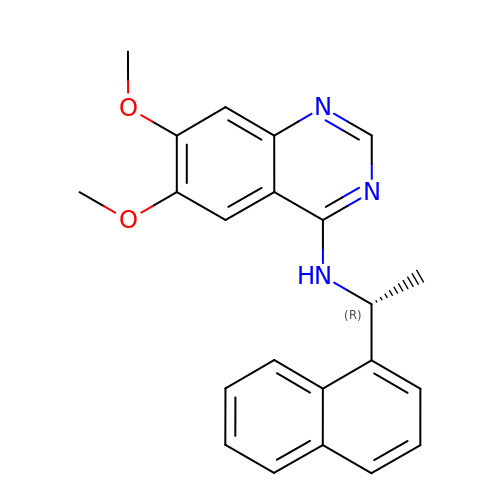6,7-dimethoxy-~{N}-[(1~{R})-1-naphthalen-1-ylethyl]quinazolin-4-amine | C22 H21 N3 O2 | YREPTYNUQVYXCF-CQSZACIVSA-N>[2x]MHHHHHHTSLYKKAGFLVPRGSEDRDPTQFEERHLKFLQQLGKGNFGSVEMCRYDPLQDNTGEVVAVKKLQHSTEEHLRDFEREIEILKSLQHDNIVKYKGVCYSAGRRNLKLIMEYLPYGSLRDYLQKHKERIDHIKLLQYTSQICKGMEYLGTKRYIHRDLA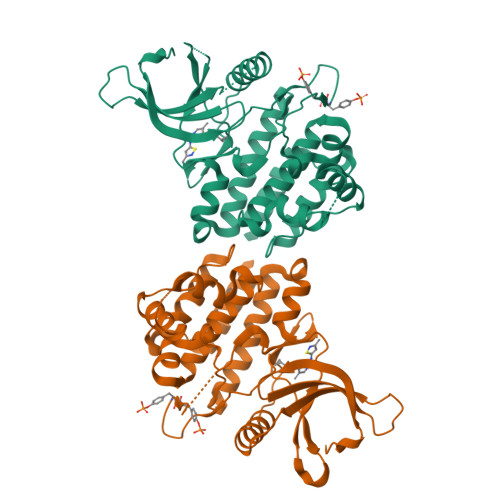TRNILVENENRVKIGDFGLTKVLPQDKEYYKVKEPGESPIFWYAPESLTESKFSVASDVWSFGVVLYELFTYIEKSKSPPAEFMRMIGNDKQGQSIVTHLIELLKNNGRLPRPDGCPDEIYMIMTECWNNNVNQRPSFRDLALRVDQIRDNMAG> NLSDFKVATWNLQGSSAVNESKWNINVRQLLSGEQGADILMVQEAGSLPSSAVRTSRVIQHGGTPIEEYTWNLGTRSRPNMVYIYYSRLDVGANRVNLAIVSRRQADEAFIVHSDSSVLQSRPAVGIRIGTDVFFTVHALATGGSDAVSLIRNIFTTFNSSSSPPERRVYSWMVVGDFNRAPANLEVALRQEPAVSENTIIIA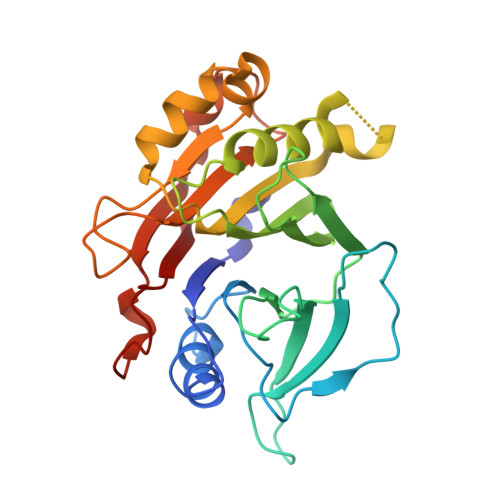PTEPTHRSGNILDYAILHDAHLPRREQARERIGASLMLNQLRSQITSDHFPVSFVRDR> SDGTWQGKQYLKEDGSQAANEWVFDTHYQSWFYIKADANYAENEWLKQGDDYFYLKSGGYMAKSEWVEDKGAFYYLDQDGKMKRNAWVGTSYVGATGAKVIEDWVYDSQYDAWFYIKADGQHAEKEWLQIKGKDYYFKSGGYLLTSQWINQAYVNASGAKVQQGWLFDKQYQSWFYIKENGNYADKEWIFENGHYYYLKSGGYMAANEWIWDKESWFYLKFDGKIAEKEWVYDSHSQAWYYFKSGGYMAANEWIWDKES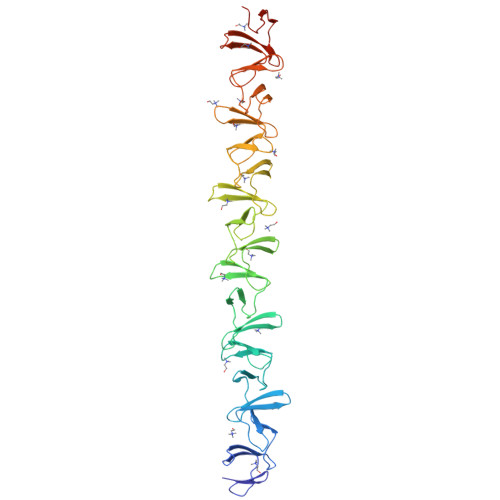WFYLKFDGKMAEKEWVYDSHSQAWYYFKSGGYMTANEWIWDKESWFYLKSDGKIAEKEWVYDSHSQAWYYFKSGGYMTANEWIWDKESWFYLKSDGKMAEKEWVYDSHSQAWYYFKSGGYMAKNETVDGYQLGSDGKWLGGKATNK> STSAGPTVPDRDNDGIPDSLEVEGYTVDVKNKRTFLSPWISNIHEKKGLTKYKSSPEKWSTASDPYSDFEKVTGRIDKNVSPEARHPLVAAYPIVHVDMENIILSKNEDQSTQNTDSQTRTISKNTSTSRTHTSEVHGNAEVHASFFDIGGSVSAGFSNSNSSTVAIDHSLSLAGERTWAETMGLNTADTARLNANIRYVNTGTAPIYNVLPTTSLVLGKNQTLATIKAKENQLSQILAPNNYYPSKNLAPIALNAQDDFSSTPITMNYNQFLELEKTKQLRLDTDQVYGNIATYNFENGRVRVDTGSNWSEVLPQIQETTARIIFNGKDLNLVERRIAAVNPSDPLETTKPDMTLKEALKIAFGFNEPNGNLQYQGKDITEFDFNFDQQTSQNIK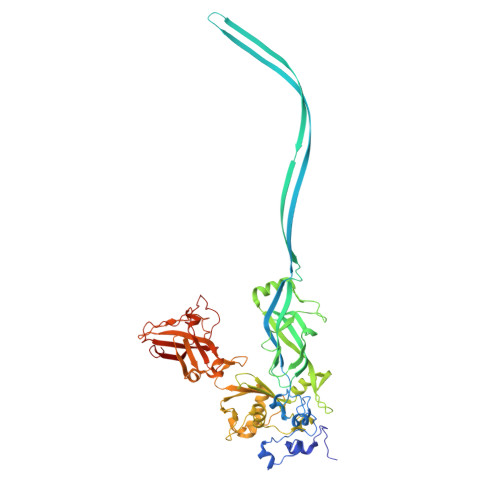NQLAELNATNIYTVLDKIKLNAKMNILIRDKRFHYDRNNIAVGADESVVKEAHREVINSSTEGLLLNIDKDIRKILSGYIVEIEDTEGLKEVINDRYDMLNISSLRQDGKTFIDFKKYNDKLPLYISNPNYKVNVYAVTKENTIINPSENGDTSTNGIKKILIFSKKGYEIG Pyrrolo-dC | C12 H15 N3 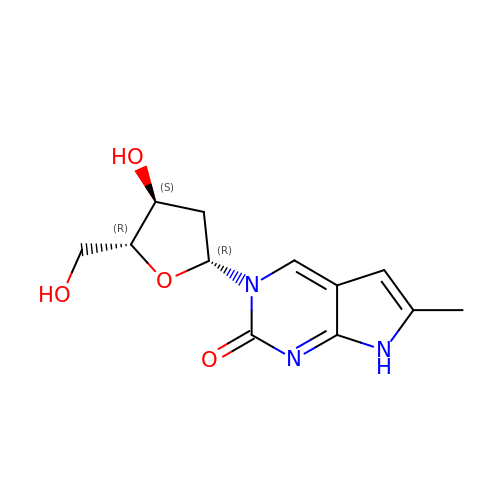O4 | NMRPZKUERWKZCL-IVZWLZJFSA-N> VD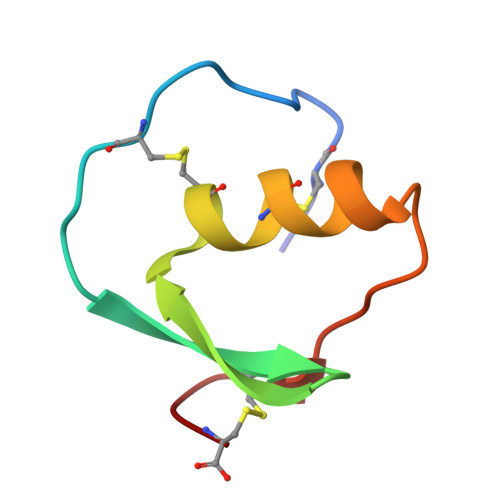CSEYPKPACTPEYRPLCGSDNKTYGNKCNFCNAVVESNGTLTLSHFGKC>[2x]GPLGSTEADSQQASTLPDLAEQFAPPDVAPPLLIKLVEAIEKKGLECSTLYRTQSSSNPAEL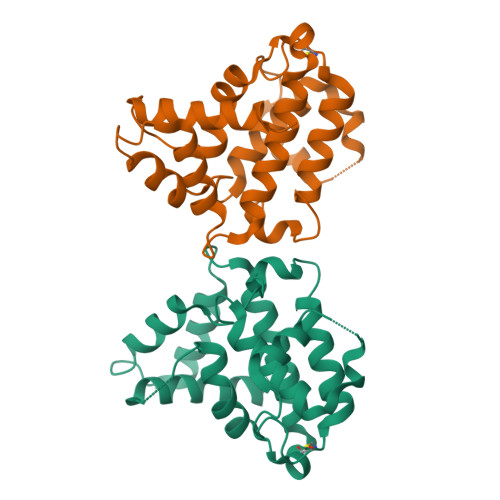RQLLDCDTASLDLEMFDVHVLADAFKRYLLDLPNPVIPVAVSSELISLAPEVQSSEEYIQLLKKLIESPSIPHQYWLTLQYLLKHFFKLSQTSSKNLLNARVLSELFSPLLFRFPAASSENTEHLIKIIEILISTEWNERQPAPALPPKPPKPTTVAN>[2x]GAMEVEVKLRLLTAAAHLRLTTLLTPYHLKTLHQRNTFFDTPKNDLSLRRAVLRLRFLQNAAVSAASPSPPRCIVSLKAKPTLANGISRVEEDEEEIEYWIGKECVESPAKLSDIGSRVLKRVKEEYGFNDFLGFVCLGGFENVRNVYEWRGVKLEVDETKYDFGNCYEIECETEEPERVKTMIEEFLTEEKIEFSNSDMTKFAVFRSGKLP

The Vtc4p β-tunnel domain is not unique to eukaryotic polyP polymerases but is a structural hallmark of triphosphate tunnel metalloenzymes (TTMs), whose characteristic features are the presence of a topologically closed hydrophilic β-barrel, the preference for triphosphate-containing substrates, and for a divalent metal co-factor (PFAM families CYTH and VTC). Members of the ancient triphosphate tunnel metalloenzyme family can be found in all kingdoms of life. Our comparative analysis defines that most of these enzymes share a common catalytic mechanism in their tunnel centers, yet they have evolved different substrate recognition modes on their tunnel entries. The observed substrate plasticity apparently allows TTM proteins to act on a wide array of enzyme substrates and to perform very different reactions, many of which likely remain to be discovered.

We determined co-crystal structures of AtTTM3 with tripolyphosphate and Mg2+ or Mn2+ metal co-factors in two independent crystal lattices. As AtTTM3 efficiently hydrolyzes PPPi in the presence of Mg2+ ions only at neutral or basic pH, we used two crystal forms grown at pH 5.0 (form A) and pH 7.5 (form B) to crystallize substrate-metal complexes under non-hydrolyzable and hydrolyzable conditions, respectively. In both crystal forms, we determined structures of AtTTM3 in the presence of PPPi and either MgCl2 or MnCl2. At pH 5.0 (form A) we find a triphosphate moiety bound in the AtTTM3 active site. Here, PPPi coordinates a Mg2+/Mn2+ ion that acts as a bridge between the substrate and the invariant Glu-169AtTTM3. The same metal co-factor coordination has been previously found in a Vtc4p AppNHp-Mn2+ complex. In all our structures the catalytic Mg2+ ions can be substituted by Mn2+ ions, for which we calculated phased anomalous difference electron density maps from data collected near the Mn-K edge to confirm their modeled positions. Comparison of AtTTM3 and Vtc4p revealed that four basic residues, which lead the growing polyP chain away from the active site in Vtc4p, are specifically replaced by four glutamate residues (Glu-2AtTTM3, Glu-4AtTTM3, Glu-90AtTTM3, and Glu171AtTTM3) in AtTTM3. These residues, which form an acidic patch in the vicinity of the AtTTM3 tripolyphosphate substrate, are conserved among diverse TTM proteins with different catalytic activities.>[2x]MTIFQFPQDFMWGTATAAYQIEGAYQEDGRGLSIWDTFAHTPGKVFNGDNGNVACDSYHRYEEDIRLMKELGIRTYRFSVSWPRIFPNGDGEVNQKGLDYYHRVVDLLNDNGIEPFCTLYHWDLPQALQDAGGWGNRRTIQAFVQFAETMFRE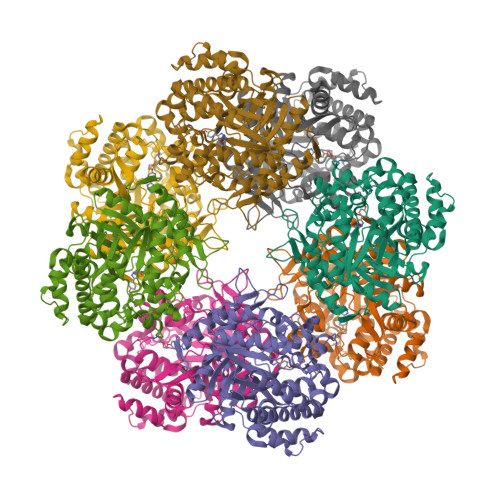FHGKIQHWLTFNEPWCIAFLSNMLGVHAPGLTNLQTAIDVGHHLLVAHGLSVRRFRELGTSGQIGIAPNVSWAVPYSTSEEDKAACARTISLHSDWFLQPIYQGSYPQFLVDWFAEQGATVPIQDGDMDIIGEPIDMIGINYYSMSVNRFNPEAGFLQSEEINMGLPVTDIGWPVESRGLYEVLHYLQKYGNIDIYITENGACINDEVVNGKVQDDRRISYMQQHLVQVHRAIHDGLHVKGYMAWSLLDNFEWAEGYSMRFGIIHVDFRTQVRTPKESYYWYRKVVGNNWLETRR Human excitatory amino acid transporters (EAATs) concentrate the neurotransmitter glutamate and aspartate in cells. By coupling the uptake of one substrate molecule to movements of five ions—symport of three sodium (Na+) ions and a proton and countertransport of one potassium (K+) ion—EAATs ensure that the cytoplasmic glutamate concentration is ~10 mM, which is required for neuronal functions, while the extracellular concentrations are as low as a few nM permitting rounds of synaptic signaling. EAATs are homotrimers composed of promoters that work independently. TMs 1, 2, 4, and 5 of each protomer comprise the scaffold domain mediating trimerization; TMs 3, 6, 7, and 8 and helical hairpins (HPs) 1 and 2 form the substrate-binding transport domain.

EAAT3-X was predominantly found in OFS in NaCl buffer and iOFS in NMDG, NaCl/glutamate, and KCl buffers. Notably, we observed no K+ ions bound in OFS determined in KCl buffer and assigned the state as apo (described in detail below). Surprisingly, when we examined the OFS conformations imaged in the NMDG chloride and KCl buffers, we found that they closely resembled OFS-Na+ with wide-open HP2 gates. We observed no density in the K+-binding site, suggesting that potassium did not bind to OFS even though it was present at 300 mM. We term these nearly identical structures (RMSD 0.57 Å) OFS-ApoNMDG and OFS-ApoK and refer to them collectively as OFS-Apo for short. Strikingly, the YE/DDR motifs of OFS-Apo are in the bound configuration, while their NMD motifs are in a configuration intermediate between apo and bound conformations. Inspection of the Na3 sites in OFS-ApoNMDG and OFS-ApoK revealed distorted geometries of the ion-coordinating residues, including shifted N366 sidechains. We found excess nonprotein densities at the sites, likely due to water molecules. In contrast, in OFS-Apo and OFS-Na+, E374 is buried and proximal to G415. It is likely protonated with pKa-s of 9.2, 10.0, and 7.6 for OFS-ApoK, OFS-ApoNMDG, and OFS-Na+, respectively. OFS-Apo features an open HP2, protonated E374, and bound-like NMD and YE/DDR motifs.

> GPMGKPARKGAEWKRFLKNNWVLLSTVAAVVLGITTGVLVREHSNLSTLEKFYFAFPGEILMRMLKLIILPLIISSMITGVAALDSNVSGKIGLRAVVYYFATTLIAVILGIVLVVSIKPGVTQKVGEIARTGSTPEVSTVDAMLDLIRNMFPENLVQAAFQQYKTKREEVKPPSDPEMTMTEESFTAVMTTAISKTKTKEYKIVGMYSDGINVLGLIVFALVFGLVIGKMGEKGQILVDFFNALSDATMKIVQIIMWYMPLGILFLIAGCIIEVEDWEIFRKLGLYMATVLTGLAIHSIVILPLIYFIVVRKNPFRFAMGMAQALLTALMISSSSATLPVTFRCAEENNQVDKRITRFVLPVGATINMDGTALYEAVAAVFIAQLNDLDLGIGQIITISITATSASIGAAGVPQAGLVTMVIVLSAVGLPAEDVTLIIAVDCLLDRFRTMVNVLGDAFGTGIVEKLSKKELEQMDVSSEVNIVNPFALESTILDNEDSDTKKSYVNGGFAVDKSDTISFTQTSQF> ADTLLILGDSLSAGYRMSASAAWPALLNDKWQSKTSVVNASISGDTSQQGLARLPALLKQHQPRWVLVELGGNDGLRGFQPQQTEQTLRQILQDVKAANAEPLLMQIRPPANYGRRYNEAFSAIYPKLAKEFDVPLLPFFMEEVYLKPQWMQDDGIHPNRDAQPFIADWMAKQLQPLVNHDSLEHH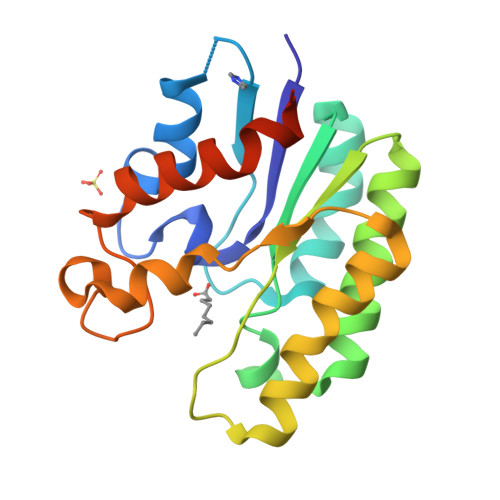HHHH> MSLSSWRQFQLFENIPIRDPNFGGDSLLYSDPTLCAATIVDPQTLIIAVNSNIIKVVKLNQSQVIHEFQSFPHDFQITFLKVINGEFLVALAESIGKPSLIRVYKLEKLPNREQLYHSQVELKNGNNTYPISVVSISNDLSCIVVGFINGKIILIRGDISRDRGSQQRIIYEDPSKEPITALFLNNDATACFAATTSRILLFNTTGRNRGRPSLVLNSKNGLDLNCGSFNPATNEFICCLSNFIEFFSSSGKKHQFAFDLSLRKRIFCVDKDHILIVTEETGVPTTSISVNELSPTIINRIFIIDAKNKIISLNFVVSSAIIDIFSTSQSGKNITYLLTSEGVMHRITPKSLENQINIIIQKELYPFALQLAKQHSLSPLDVQEIHKKYGDYLFKKGLRKEATDQYIQCLDVVETSEIISKFGVKEVPDPESMRNLADYLWSLIKNSISQRDHVTLLLIVLIKLKDVEGIDTFIQHFDRKGIWNEGVVMDDMDDVTFFYSDNDFFDLDLILELMKESDFKRLSYRLAKKYSKDSLIIVDILLNLLHNPVKAIKYIKSLPIDETLRCLVTYSKKLLEESPNETNALLIEVFTGKFKPSTFEVDLDRRDTTGDFSENIRTVFYSYKTFFNYMNSNGTSDAMSESSEASHEHEEPTYHPPKPSIVFSSFVTKPFEFVVFLEACLACYQQYEGFDEDRQVILTTLYDLYLNLAQNDVPERIDDWRSRATGVLRESNKLVYSAASNNTSKRVDNSIMLLISHMDQSSASAKDKTKIDIASFANDNPEMDLLSTFRAMTLNEEPSTCLKFLEKYGTEEPKLLQVALSYFVSNKLIFKEMGGNEVLKEKVLRPIIEGERMPLLDIIKALSRTNVAHFGLIQDIIIDHVKTEDTEIKRNEKLIESYDKELKEKNKKLKNTINSDQPLHVPLKNQTCFMCRLTLDIPVVFFKCGHIYHQHCLNEEEDTLESERKLFKCPKCLVDLETSNKLFEAQHEVVEKNDLLNFALNSEEGSRDRFKVITEFLGRGAISYSDITI;> MKNPSFDWERLKDVFYRSRAIGELKWPTQYEEFKCALSLTVIAVEIQDFIQVYNYFGQLLGKINLQRIHEDIIKFEFDKDEKLILVTKSSIKIVKGWSPLTIESVPLQDPTIDTIWDYHNGIMLLAKSRDIYKLNGNEWELLYENKDKKYNLLTKNHWSCNDDSIILLDVDHVYQVSTSNGALLKLITDSSWHKVTISSRGFICLYNMKDNKLQIFRDPARILMEHNLDSTPDDICWCGNDTVACSFEDEIKLYGPDGLYVTFWYPFTVTNLRAEVDGLKVITTEKIYFLSRVQPQTSNIFRIGSTEPGAMLVDSFSLLEDHAPKAIEILKNFVLEKGVLDCIAAAIDEFEPKLQKMLLNAASYGKASLQYKSFDASIFVNACNTIKLLNCFRSFGIFLTVEEYRCISLKGVIDRLLKYHRYYECIQICKLANERFLLGYVFTEWAKDKIKGSPDMEDDELLDKIKSRLSVIDMTDTLQMVAVAKVAYLEGRFQLSRNLALLEKNEEARIEQLYNLDDDSIALKECIKVQNYSLTISLLIALSKKLTNSQLTKLLIIDMFNNPLYLYYMRMDKAYLYDFYRQTDRFIDLAHVLLQQGKEQQSLHSFLPQIKDLYSQVQNSEVVNNTIEQLQRQEKLWIYQESLGKRFAISFTNMTLDQTLSKLIETGQDKQVKEIVKKFKISEKKLYHLKCKTLVEAKKFDELLQFAQSRKSPIGYMPFYTYLKSRGHMDKASPYVNMIPGLSYQEKKKLYVECRGFRDAIQLAGKEKDIPGLKEIYNIIPPNEPELKALANETMSRI;> MIKTRIEEVQLQFLTGNTELTHLKVSNDQLIVTTQRTIYRINLQDPAIVNHFDCPLSKELETIMNVHVSPMGSVILIRTNFGRYMLLKDGEFTQLNKIKNLDLSSLHWINETTFLMGIKKTPKLYRVELTGKDITTKLWYENKKLSGGIDGIAYWEGSLLLTIKDNILYWRDVTNMKFPLVLPDESEQFERLKHHAIKKFDSYNGLFAWVTSNGIVFGDLKEKQMEKDPASNNFGKFLSSSKVLLNFELPDYQNDKDHLIKDIVLTAFHILLLRKNTVTMVSQLNNDVVFHETIPRHQLTGSNTDSNEKFLGLVRDSVKETFWCFSNINVFEIIIENEPNSVWNLLVRDNKFDKALSLKGLTVREIESVKLSKAMYLFHTAKDFHSAAQTLGSMKDLSHFGEIALNFLQIKDYNDLNVILIKQLDNVPWKSTQVVLSSWIIWNFMKQLNDIELKINTTKPASTDEDNLLNWNLNLKEKSNELTKFLESHLEKLDNETVYQIMSKQNRQNELLIFASLINDMKFLLSFWIDQGNWYESLKILLTINNHDLVYKYSLILLLNSPEATVSTWMKIKDLDPNKLIPTILKFFTNWQNNSKLITNISEYPENYSLTYLKWCVREVPKMCNPIVYNSILYMMITDPRNDMILENDIIKFMKSNENKYDLNFQLRLSLKFKKTKTSIFLLTRLNLFEDAIDLALKNNLIDDCKVIVNDEILIEDYKLRKRLWLKIAKHLLLSMKDIDIKQLIRTILNDSNEILTIKDLLPFFNEYTTIANLKEELIKFLENHNMKMNEISEDIINSKNLKVEINTEISKFNEIYRILEPGKSCDECGKFLQIKKFIVFPCGHCFHWNCIIRVILNSNDYNLRQKTENFLKAKSKHNLNDLENIIVEKCGLCSDININKIDQPISIDETELAKWNE;> MNRFWNTKKFSLTNADGLCATLNEISQNDEVLVVQPSVLPVLNSLLTFQDLTQSTPVRKITLLDDQLSDDLPSALGSVPQMDLIFLIDVRTSLRLPPQLLDAAQKHNLSSLHIIYCRWKPSFQNTLEDTEQWQKDGFDLNSKKTHFPNVIESQLKELSNEYTLYPWDLLPFPQIDENVLLTHSLYNMENVNMYYPNLRSLQSATESILVDDMVNSLQSLIFETNSIITNVVSIGNLSKRCSHLLKKRIDEHQTENDLFIKGTLYGERTNCGLEMDLIILERNTDPITPLLTQLTYAGILDDLYEFNSGIKIKEKDMNFNYKEDKIWNDLKFLNFGSIGPQLNKLAKELQTQYDTRHKAESVHEIKEFVDSLGSLQQRQAFLKNHTTLSSDVLKVVETEEYGSFNKILELELEILMGNTLNNDIEDIILELQYQYEVDQKKILRLICLLSLCKNSLREKDYEYLRTFMIDSWGIEKCFQLESLAELGFFTSKTGKTDLHITTSKSTRLQKEYRYISQWFNTVPIEDEHAADKITNENDDFSEATFAYSGVVPLTMRLVQMLYDRSILFHNYSSQQPFILSREPRVSQTEDLIEQLYGDSHAIEESIWVPGTITKKINASIKSNNRRSIDGSNGTFHAAEDIALVVFLGGVTMGEIAIMKHLQKILGKKGINKRFIIIADGLINGTRIMNSIS;> MVKKKTNNDKGKEVKENEGKLDIDSESSPHERENDKKKTEDDSLRATESEETNTHNANPNETVRADKFSQEESRPIEDSPHTDKNTAQESCQPSSAEDNVINTDITSLNEKTSTNDEQEKGLPLKISEGPFTISTLLDNVPSDLIYTCCEAYENHIFLGTTTGDLLHYFELERGNYMLVSQTKFDAESNSKIDKILLLPKVEGALILCDNELVLFILPEFAPRPNTTRLKGISDVVICNFSRSSKAYRIYAFHAEGVRLLKISADSLVLTKAFNFKLIDKACAHEETLMVSKLNSYELINLKSSQVIPLFRISETDEDLEPIITSFNEQSEFLVCSGGGSYDSGAMALVVNHHGDIIKGTIVLKNYPRNVIVEFPYIIAESAFQSVDIYSALPSEKSQLLQSITTSGSDLKISKSDNVFTNTNNSEEFKEKIFNKLRLEPLTHSDNKFRIERERAFVEESYEEKTSLIVYNNLGIHLLVPTPMVLRFTSCEESEIDNIEDQLKKLAKKDLTKFEHIEAKYLMSLLLFLMTLHYDHIEDEVMKKWCDFSDKVDIRILFYMFGWKVYSEIWCFHGLINIVERLKSLKLTNKCENILKMLLMMKNELKKKNKTGLLTNDFDDIMKTIDITLFKLRLEKKETITVDMFERESYDEIIREINLHDDKLPRIELLIEIYKEKGEYLKALNLLREAGDYISLVSFIEENLKKLPEDYIKERIADDLLLTLKQGDENTEECAIKKVLKILDMACINKNDFLNKIPAEETSLKVSFIEQLGVQNSNDSKFLFNYYLAKLREIINQSNIWSILGDFIKEYKDDFAYDKTDITNFIHIKLKHSLQCENFSKYYEKCENLKSENEKDDEFINFTFDEISKIDKEHILTLLFFPNELTNWVSSEELLKIYLSFNDFRSVEKYIGKQNLVAVMKQYLDISSLNYSVELVTNLLQRNFELLDDTDIQLKILETIPSVFPVQTISELLLKVLIKYQEKKEESNLRKCLLKNQISISDELSRNFDSQG;> MEQNGLDHDSRSSIDTTINDTQKTFLEFRSYTQLSEKLASSSSYTAPPLNEDGPKGVASAVSQGSESVVSWTTLTHVYSILGAYGGPTCLYPTATYFLMGTSKGCVLIFNYNEHLQTILVPTLSEDPSIHSIRSPVKSIVICSDGTHVAASYETGNICIWNLNVGYRVKPTSEPTNGMTPTPALPAVLHIDDHVNKEITGLDFFGARHTALIVSDRTGKVSLYNGYRRGFWQLVYNSKKILDVNSSKEKLIRSKLSPLISREKISTNLLSVLTTTHFALILLSPHVSLMFQETVEPSVQNSLVVNSSISWTQNCSRVAYSVNNKISVISISSSDFNVQSASHSPEFAESILSIQWIDQLLLGVLTISHQFLVLHPQHDFKILLRLDFLIHDLMIPPNKYFVISRRSFYLLTNYSFKIGKFVSWSDITLRHILKGDYLGALEFIESLLQPYCPLANLLKLDNNTEERTKQLMEPFYNLSLAALRFLIKKDNADYNRVYQLLMVVVRVLQQSSKKLDSIPSLDVFLEQGLEFFELKDNAVYFEVVANIVAQGSVTSISPVLFRSIIDYYAKEENLKVIEDLIIMLNPTTLDVDLAVKLCQKYNLFDLLIYIWNKIFDDYQTPVVDLIYRISNQSEKCVIFNGPQVPPETTIFDYVTYILTGRQYPQNLSISPSDKCSKIQRELSAFIFSGFSIKWPSNSNHKLYICENPEEEPAFPYFHLLLKSNPSRFLAMLNEVFEASLFNDDNDMVASVGEAELVSRQYVIDLLLDAMKDTGNSDNIRVLVAIFIATSISKYPQFIKVSNQALDCVVNTICSSRVQGIYEISQIALESLLPYYHSRTTENFILELKEKNFNKVLFHIYKSENKYASALSLILETKDIEKEYNTDIVSITDYILKKCPPGSLECGKVTEVIETNFDLLLSRIGIEKCVTIFSDFDYNLHQEILEVKNEETQQKYLDKLFSTPNINNKVDKRLRNLHIELNCKYKSKREMILWLNGTVLSNAESLQILDLLNQDSNFEAAAIIHERLESFNLAVRDLLSFIEQCLNEGKTNISTLLESLRRAFDDCNSAGTEKKSCWILLITFLITLYGKYPSHDERKDLCNKLLQEAFLGLVRSKSSSQKDSGGEFWEIMSSVLEHQDVILMKVQDLKQLLLNVFNTYKLERSLSELIQKIIEDSSQDLVQQYRKFLSEGWSIHTDDCEICGKKIWGAGLDPLLFLAWENVQRHQDMISVDLKTPLVIFKCHHGFHQTCLENLAQKPDEYSCLICQTESNPKIVDYKDDDDKDYKDDDDKDYKDDDDK

The hexameric HOPS and CORVET are evolutionarily conserved tethering complexes within the endolysosomal system of eukaryotic cells. Early endosome fusion is promoted by the Rab5 GTPase and its effector, the hexameric CORVET tethering complex, which is homologous to the lysosomal HOPS. Vps11 and Vps18 form the central core to which Vps33 and Vps16 are attached as an SM module to promote SNARE assembly. The two unique subunits determine the respective Rab specificity of the tethering complexes.

CORVET was produced in yeast cells and isolated via a FLAG tag on Vps8 using affinity chromatography followed by size exclusion chromatography (SEC) with high purity. From 33882 micrographs, 219391 selected particles provided a consensus map with 4.6 Å resolution. Local refinements further improved the resolution to 3.8 Å (SNARE-binding module). CORVET and HOPS share strong structural homology. Their respective cores, consisting of identical subunits (Vps11 and Vps18), are virtually indistinguishable from each other. Vps3 and Vps8 are specific to CORVET and located at the distal ends of the complex. Similarly, to the analogous subunit Vps39 in HOPS, the C-terminal α-helix of Vps3 is anchored to CORVET’s core through an interaction with the RING finger domain and the long α-helix located at the C-terminus of Vps11. In contrast, the CORVET subunit Vps3 lacks any further C-terminal extensions after the long α-helix, thus significantly reducing the contact area in the Vps3-Vps11 interface. Vps8 exhibits a characteristic elbow configuration, which turns its N-terminal half towards the β-propeller of Vps11. Moreover, a hairpin protruding from the Vps8 RING finger domain is sandwiched in a hydrophobic groove between Vps33 and Vps18, clamping the SNARE-binding unit from both sides together with the C-terminus of Vps18. In addition to the C-terminal interaction with Vps18, and distinctive from HOPS, the α-solenoid of Vps8 has two additional interfaces with Vps11.> MVKVDLESKRYGEKLKEVFLMLDNNVVECIKEITESSRNGKLVFFVGAGVSTLSDYPQWWRLVDKYHEELYGSPKKGNYSSDEYLRIPQIFYNVKGEMAFDGILKDFFQVDKPTNPIHDKILAMNPAHVITTAYDNLIDTACWKRGKYFSVISAEEDVANATSSRYLLKVAGDFRKGFKGENVVLKEDDYLNYDQNYPLISNLMKTIIATHTIVFIGYGLGDYNINMLLNWVRKLQKDSFHKPFFIRTDPSPIENETLIYYENKGLRIIDAASLIDSNEYDYLERYSAVMDLLIESQENKFITKDDEVIDYIYGKISPLFALQYIRKIDLKHVFEYDYHFEVNGTVVRHKNKGFGYMERFFELKESCDERSKLSKKQYERFNALFNFFEKNGVICMAKDAGTLNTSIEINSLAYHGKYDVMKKFIEEQSVSIEDDYKKAFFLACLGRWEESYDLYSNIILNSIDESNGCVYYLSQINRYRIYQSITQAVTQFNGLGLLTFGRHYKPFTDEF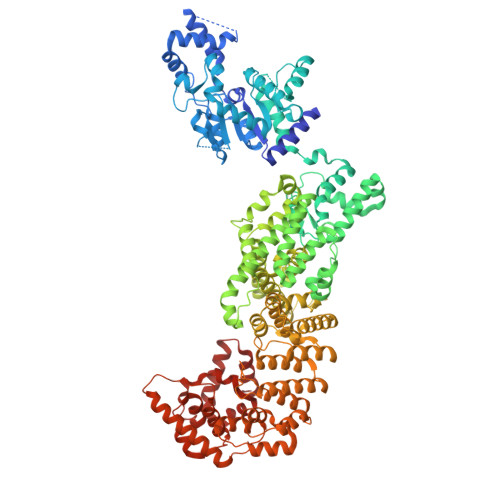LARIEREMTNFNIDDLFNGMPFEFQKKYKILEFLSDNQFLYDDTVKLFELTNKVRSEMSEGSYSFGMSSDIVVLLRLYDNLRFLYENCLWSVSFHEFHQYIRNSMSLLIEKAEYERTRDIDELGFSFFGKKSGFFMEYYDFVNISRHFKIDDIKNLERSCSIDKIRFGEQEKIEEYLVGIAEEITKQFSANGMNVVFYTQFISEAKAALYFAKYVKLSEEGLGKIVKALLFYFPERDLDIGKRYVWLERLTKCNELPKSIISIIDDFLVLQAEKHIDQNYSEVSSNGLYSRDYGALIKHFEKNFISKRLSEITLCLTQDKQKQIDFLFKLLPLLSTNAKSHLLSFKSVENINDLMNGIRIGLIDEFTPEHEELIIEYLETRKVNYIVEKEKGIQTFSSNDYMSTFGIWYFLEEINNSKMEEFIGMDDQYDFFVDPENFDYKKFIPSWLKNYNDKLLGKIAGNKHMKHHVIEVLKERVKNSNDKRYLEILMNYFI> MMAPVQKQFREFHDRIKLAQYDENQTLRDERDAVLTAVREGLKKVFADRGEAAPTFTPFNQGSYAMNTGVKPLEGGEYDIDVGIILNIAKDDHDPVEVKKWIRDALKDYGNGAEIRRSCVTVFKPGYHVDLAVYADPELSGGTLCIAKGKENSGDEHRLWQISDPQGFQDRIASKLSGDDAAQFRRCIRYLKRWRDFRFSSDGNAAPLGIGLTAAAYWWFQVSKRTDPVSQNVTYDDRDALEQFVQTMLDNFHDTWDSKDQRSYPRLTVELPVQPYNDVFE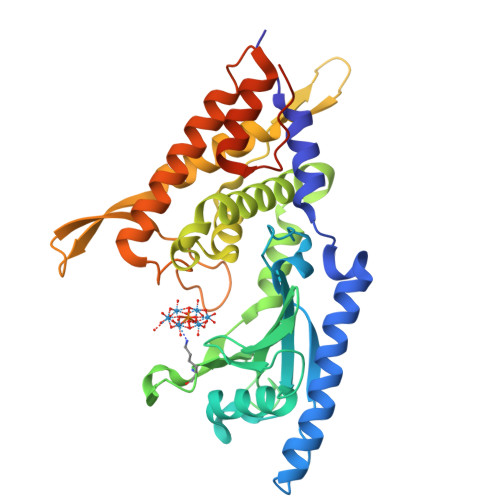KMTGMQMESFKSKLQALLNALKTAKSRLELHDACKALADHFGSEFPVPEKDKSAVHTAPAIVGSGSSG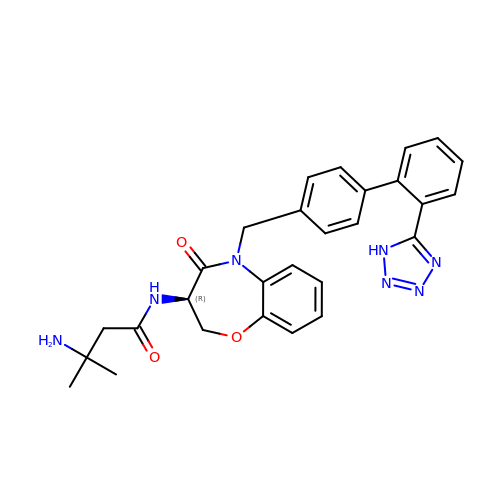3-azanyl-3-methyl-~{N}-[(3~{R})-4-oxidanylidene-5-[[4-[2-(1~{H}-1,2,3,4-tetrazol-5-yl)phenyl]phenyl]methyl]-2,3-dihydro-1,5-benzoxazepin-3-yl]butanamide | C28 H29 N7 O3 | PJFIRCYASUNIFO-JOCHJYFZSA-N>MGHHHHHHSLRDLKEENRIVIWPSYFFSPTRSKGRRLARIPYKIKTEELVSTLRELGLDPIVIENKKYPRDRKINF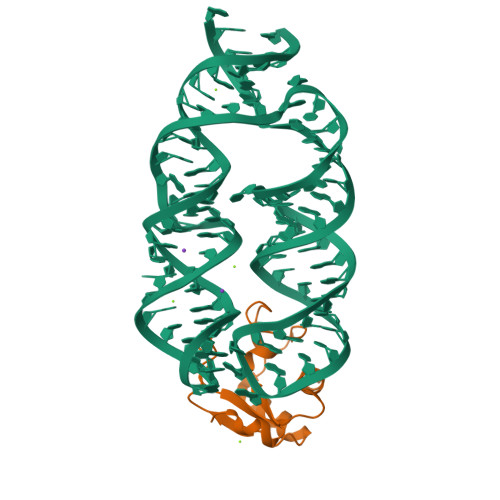LIAVKKVKSKNYTLKIIHNALMGTRQTNPNKSN[2x]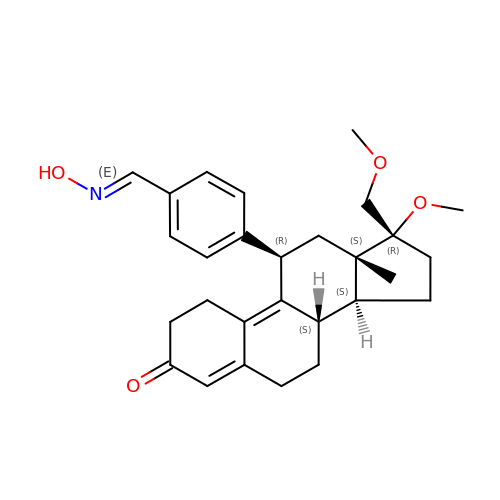4-[(11BETA,17BETA)-17-METHOXY-17-(METHOXYMETHYL)-3-OXOESTRA-4,9-DIEN-11-YL]BENZALDEHYDE OXIME | C28 H35 N O4 | GJMNAFGEUJBOCE-MEQIQULJSA-N>[4x]GAMAQELKERAKVFAKPIGASYQGILDQLDLVHQAKGRDQIAASFELNKKINDYIAEHPTSGRNQALTQLKEQVTSALFIGKMQVAQ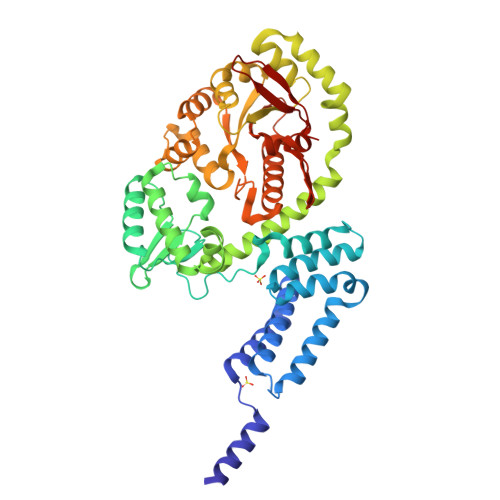AGIDAIAQTRPELAARIFMVAIEEANGKHVGLTDMMVRWANEDPYLAPKHGYKGETPSDLGFDAKYHVDLGEHYADFKQWLETSQSNGLLSKATLDESTKTVHLGYSYQELQDLTGAESVQMAFYFLKEAAKKADPISGDSAEMILLKKFADQSYLSQLDSDRMDQIEGIYRSSHETDIDAWDRRYSGTGYDELTNKLASATGVDEQLAVLLDDRKGLLIGEVHGSDVNGLRFVNEQMDALKKQGVTVIGLLHLRSDLAQPLIDRYLATGVMSSELSAMLKTKHLDVTLFENARANGMRIVALDANSSARPNVQGTEHGLMYRAGAANNIAVEVLQNLPDGEKFVAIYGKALLQSHKGIEGFVPGITHRLDLPALKVSDSNQFTVEQDDVSLRV> MTAPASPSVTFTNPLAEKRADPHIFKHTDGYYYFTATVPEYDRIVLRRATTLQGLATAPETTIWTKHASGVMGAHIWAPEIHFIDGKWYVYFAAGSTSDVWAIRMYVLESGAANPLTGSWTEKGQIATPVSSFSLDATTFVVNGVRHLAWAQRNPAEDNNTSLFIAKMANPWTISGTPTEISQPTLSWETVGYKVNEGPAVIQHGGKVFLTYSASATDANYCLGMLSASASADLLNAASWTKSSQPVFKTSEATGQYGPGHNSFTVSEDGKSDILVYHDRNYKDISGDPLNDPNRRTRLQKVYWNADGTPNFGIPVADGVTPVRFSSYNYPDRYIRHWDFRARIEANVTNLADSQFRVVTGLAGSGTISLESANYPGYYLRHKNYEVWVEKNDGSSAFKNDASFSRRAGLADSADGIAFESYNYPGRYLRHYENLLRIQPVSTALDRQDATF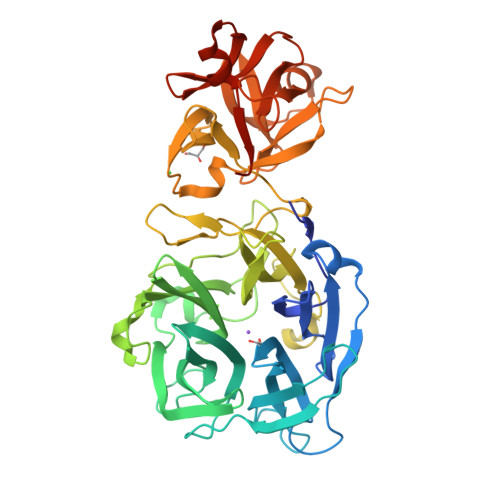YAEKLAAALEHHHHHH>[2x]MVANPEHYIKHPLQNRWALWFFKNDKSKTWQANLRLISKFDTVEDFWALYNHIQLSSNLMPGCDYSLFKDGIEPMWEDEKNKRGGRWLITLNKQQRRSDLDRFWLETLLCLIGES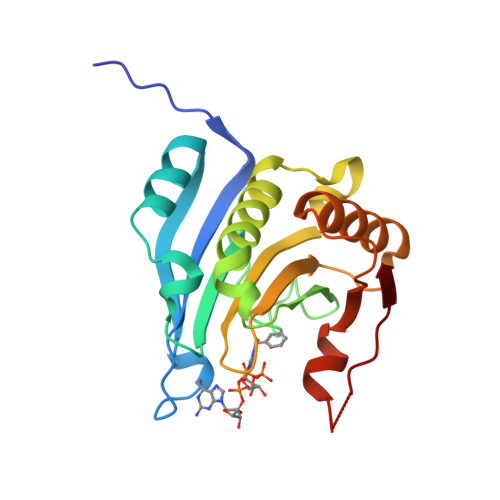FDDYSDDVCGAVVNVRAKGDKIAIWTTECENRDAVTHIGRVYKERLGLPPKIVIGYQSHADTATKSGSTTKNRFVV>MEVKIFNTQDVQDFLRVASGLEQEGGNPRVKQIIHRVLSDLYKAIEDLNITSDEYWAGVAYLNQLGANQEAGLLSPGLGFDHYLDMRMDAEDAALGIENATPRTIEGPLYVAGAPESVGYARMDDGSDPNGHTLILHGTIFDADGKPL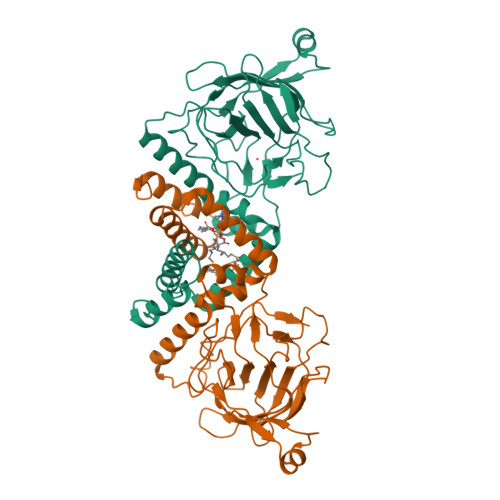PNAKVEIWHANTKGFYSHFDPTGEQQAFNMRRSIITDENGQYRVRTILPAGYGCPPEGPTQQLLNQLGRHGNRPAHIHYFVSADGHRKLTTQINVAGDPYTYDDFAYATREGLVVDAVEHTDPEAIKANDVEGPFAEMVFDLKLTRLVDGVDNQVVDRPRLAV[2x]(2S)-1-(butanoyloxy)-3-{[(R)-hydroxy{[(1r,2R,3S,4S,5R,6S)-2,3,4,5,6-pentahydroxycyclohexyl]oxy}phosphoryl]oxy}propan-2-yl tridecanoate | C26 H49 O13 P | 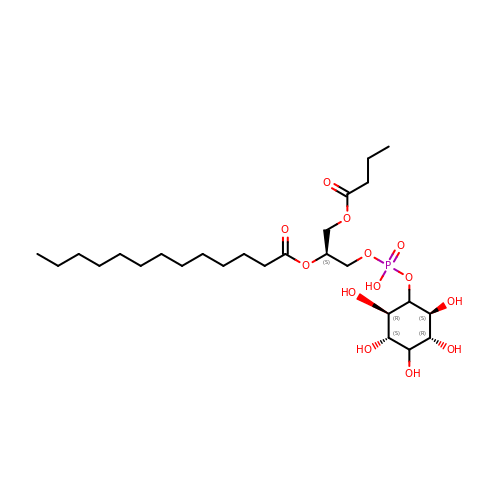PJDJYKJPFGJDMA-QYTLEKTISA-N> WSLRWRMQKSTTIAAIAGCSGAATFGGLAGGIVGCIAAGILAILQGF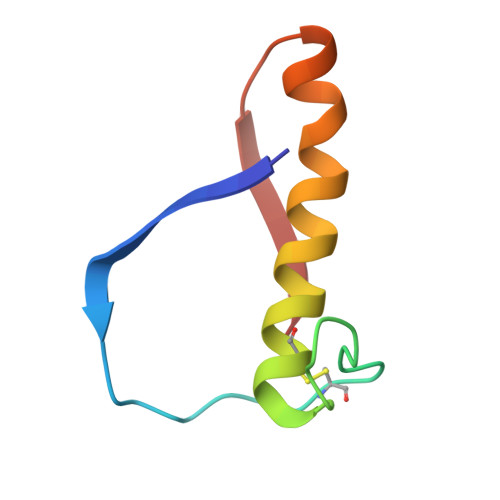EVNWHNGGGGDRSNPV> ANIVGGIEYSINNASLCSVGFSVTRGATKGFVTAGHCGTVNATARIGGAVVGTFAARVFPGNDRAWVSLTSAQTLLPRVANGSSFVTVRGSTEAAVGAAVCRSGRTTGYQCGTITAKNVTANYAEGAVRGLTQ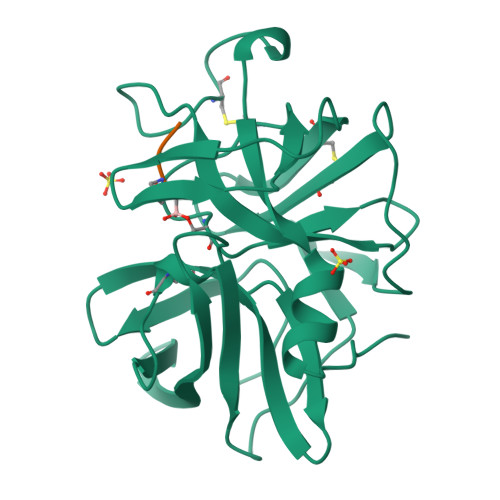GNACAGRGDSGGSWITSAGQAQGVMSGLNVQSNGNNCGIPASQRSSLFERLQPILSQYGLSLVTG;> XAAPA> PIETVPVKLKPGMDGPKVKQWPLTEEKIKALVEICTEMEKEGKISKIGPENPYNTPVFAIKKKDSTKWRKLVDFRELNKRTQDFWEVQLGIPHPAGLEKKKSVTVLDVGDAYFSVPLDEDFRKYTAF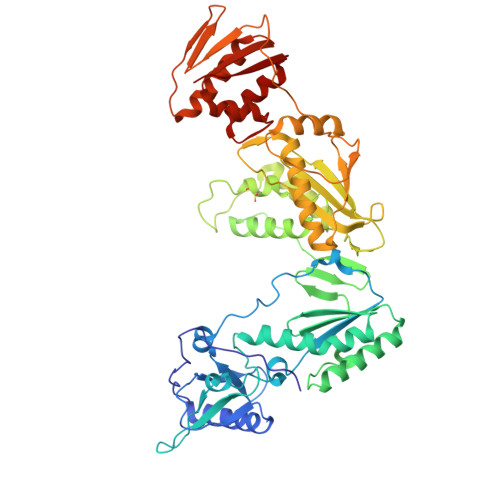TIPSINNETPGIRYQYNVLPQGWKGSPAIFQSSMTKILEPFRKQNPDIVIYQYMDDLYVGSDLEIGQHRTKIEELRQHLLRWGLTTPDKKHQKEPPFLWMGYELHPDKWTVQPIVLPEKDSWTVNDIQKLVGKLNWASQIYPGIKVRQLCKLLRGTKALTEVIPLTEEAELELAENREILKEPVHGVYYDPSKDLIAEIQKQGQGQWTYQIYQEPFKNLKTGKYARMRGAHTNDVKQLTEAVQKITTESIVIWGKTPKFKLPIQKETWETWWTEYWQATWIPEWEFVNTPPLVKLWYQLEKEPIVGAETFYVDGAANRETKLGKAGYVTNRGRQKVVTLTDTTNQKTELQAIYLALQDSGLEVNIVTDSQYALGIIQAQPDQSESELVNQIIEQLIKKEKVYLAWVP>SREFDFFTYETPKVIVVKSWTIGIINRVVQLLIISYFVGWVFLHEKAYQVRDTAIESSVVTKVKGSGLYANRVMDVSDYVTPPQGTSVFVIITKMIVTENQMQGFCPESEEKYRCVSDSQCGPERLPGGGILTGRCVNYSSVLRTCEIQGWCPTEVDTVETPIMMEAENFTIFIKNSIRFPLFNFEKGNLLPNLTARDMKTCRFHPDKDPFCPILRVGDVVKFAGQDFAKLARTGGVLGIKIGWVCDLDKAWDQCIPKYSFTRLD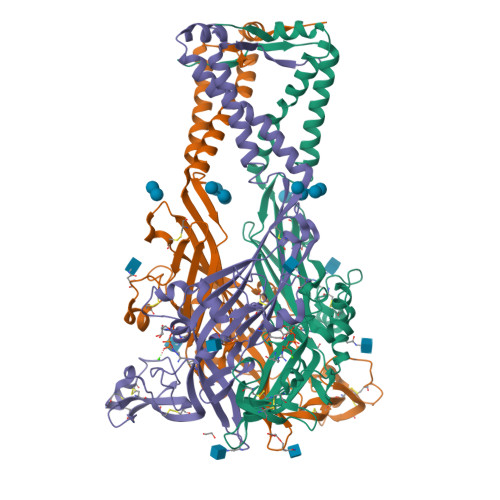SVSEKSSVSPGYNFRFAKYYKMENGSEYRTLLKAFGIRFDVLVYGNAGKFNIIPTIISSVAAFTSVGVGTVLCDIILLNFLKGADQYKAKKFEEVNE[3x]> MSLQVEGLSINLATIREQCGFAEAVDICLKHGITAIAPWRDQVAAIGLGEAGRIVRANGLKLTGLCRGGFFPAPDASGREKAIDDNRRAVDEAAELGADCLVLVAGGLPGGSKNIDAARRMVVEGIAAVLPHARAAGVPLAIEPLHPMYAADRACVNTLGQALDICETLGPGVGVAIDVYHVWWDPDLANQIARAGKMKAILAHHICD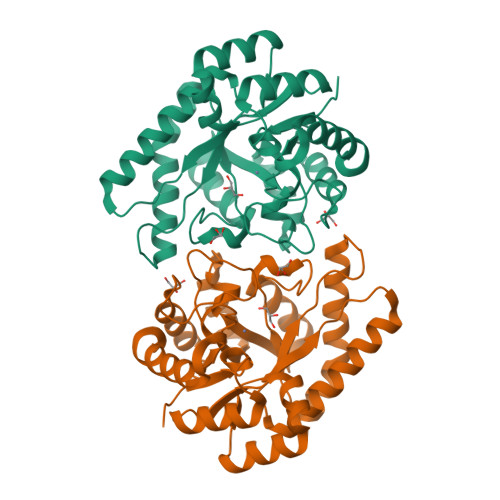WLVPTKDMLTDRGMMGDGVIDLKGIRRRIEAAGFHGAQEVEIFSADNWWKRPADEVIATCVERYRNCCEGHHHHHH> SHMP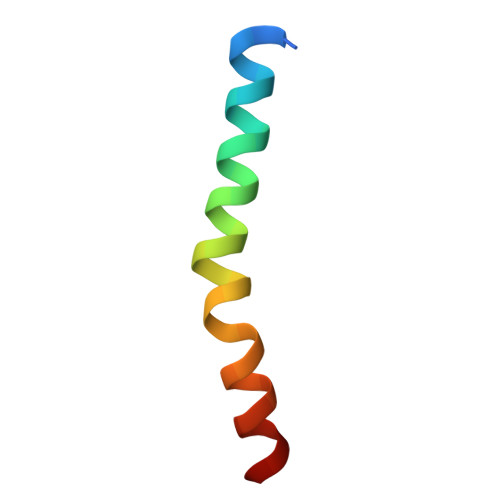RWKRHISEQLRRRDRLQRQAFEEIILQYNKLL> DKRAKVTSAMQTMLFTMLRKLDNDALNNIINNARDGCVPLNIIPLTTAAKLMVVIPDYNTY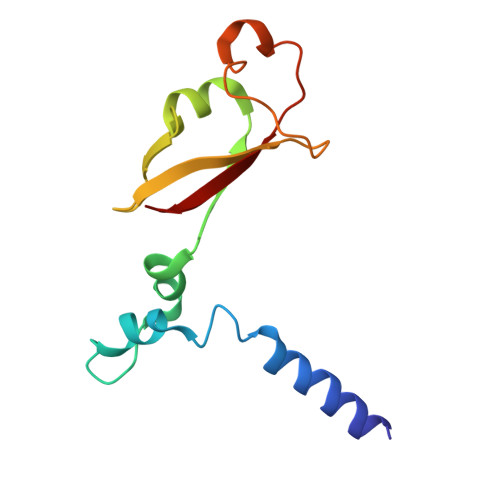KNTCDGTTFTYASALWEIQQVVDADSKIVQLSEISMDNSPNLAWPLIVTALRA>[2x]EEVVVEIRIRVQR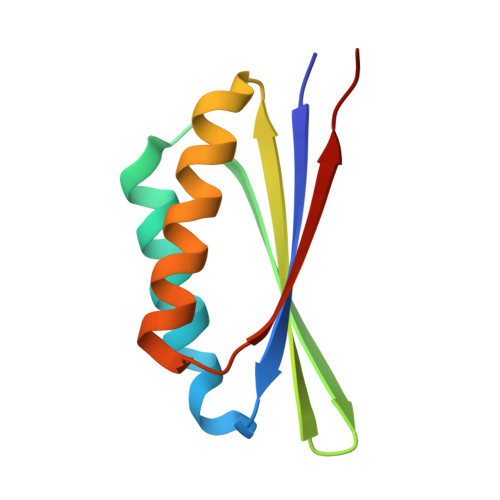EEKVRRLIKRILEEVKRESNSVEVHVETRKRNGEVEVHVRIRHDDKETIERLVERILREIKKLDKNSEVEVRTTTKR> PNFSGNWKIIRSENFEELLKVLGVNVMLRKIAVAAASKPAVEIKQEGDTFYIKTSTTVWTTEINFKVGEEFEEQTVDGRPCKSLVKWESENKMVCEQ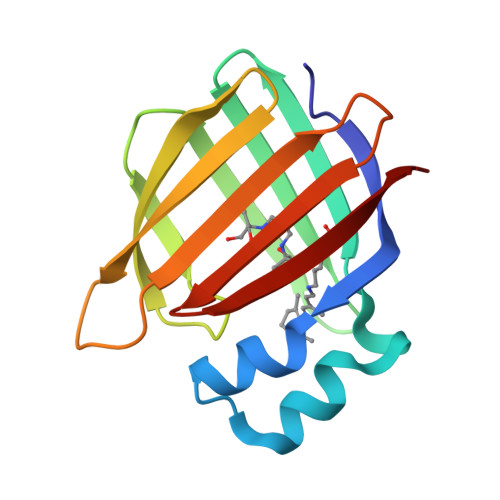KLLKGEGPKTSWTLELTNDGELIETMTADDVVCTKVYVRE> MSQRITIDPVTRIEGHLRIDCEIENGVVSKAWASGTMWRGMEEIVKNRDPRDAWMIVQRICGVCTTTHAISSVRAAESALNIDVPVNAQYIRNIILAAHTTHDHIVHFYQLSALDWVDITSALKADPAKASAMLNGVSTWHLNSAEEFTKVQNKIKDLVASGQLGIFANGCWGHPAMQLPPEVNLIAVAHYLQALECQRDANRVVALLGGKTPHIQNLAVGGVANPINLDGLGVLNLERLMYIKSFIDKLSDFVEQVYKVDTAVIAAFYPEWLERGQGAVNYLSAPEFPTD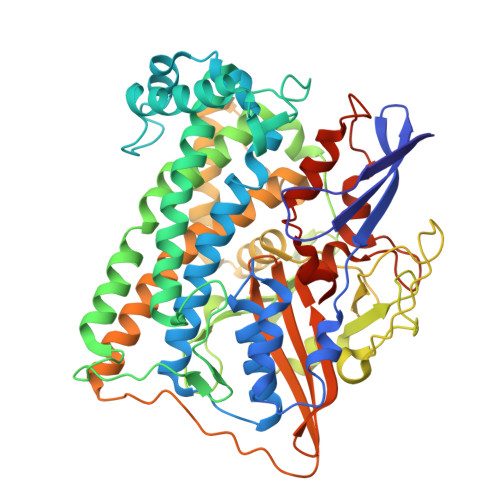GKNGSFLFPGGYITDADLSTYRPITSHSDEYLIKGIQESAKHAWYKDEAPQAPWEGTTVPDYTGWSDDGKYSWVKAPTFYGKTVEVGPLANMLCKLAAKRESTHAKLNEIVAIYTKLTGKTIEVAQLHSTLGRIIGRTVHCCELQNVLQDQYNALIVNIGKGDHTTFVKPDIPATGEFKGVGFLEAPRGMLSHWMVIKDGIISNYQAVVPSTWNSGPRNFNDEVGPYERSLVGTPIADPNKPLEVVRTIHSFDPCMSCAVHVVDVDGNEVVSVKVL> KS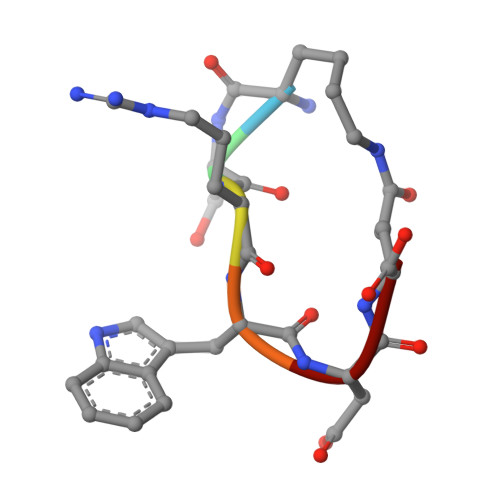RWDE>GSNQKAVIMDEQAIRRALTRIAHEIIERNKGIDGCVLVGIKTRGIYLARRLAERIEQIEGAPVPVGEIDITLYRDDLSVKTDDDEPLVKGTNVPFPVTERNVILVDDVLFTGRTVRAGMDAVMDLGRPARIQLAVLVDRGHRELPIRADFVGKNVPTSRSELIVV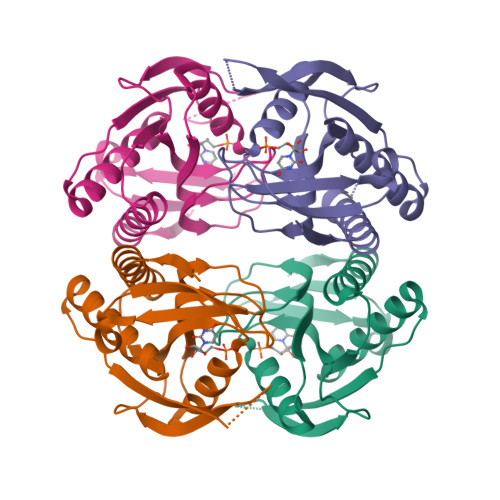ELDEVDQNDQVSIHENK[4x]>[2x]MSKAFDLVVIGAGSGGLEAGWNAATLYGKRVAVVDVQTSHGPPFYAALGGTCVNVGCVPKKLMVTGAQYMDHLRESAGFGWEFDGSSVKANWKKLIAAKNEAVLDINKSYEGMFNDTEGLDFFLGWGSLESKNVVVVRETADPKSAVKERLQADHILLATGSWPQMPAIPGIEHCISSNEAFYLPEPPRRVLTVGGGFISVEFAGIFNAYKPPGGKVTLCYRNNLILRGFDETIREEVTKQLTANGIEIMTNENPAKVSLNTDGSKHVTFESGKTLDVDVVMMAIGRIPRTNDLQLGNVGVKLTPKGGVQVDEFSRTNVPNIYAIGDITDRLMLTPVAINEGAALVDTVFGNKPRKTDHTRVASAVFSIPPIGTCGLIEEVAAKEFEKVAVYMSSFTPLMHNISGSKYKKFVAKIVTNHSDGTVLGVHLLGDGAPEIIQAVGVCLRLNAKISDFYNTIGVHPTSAEELCSMRTPSYYYVKGEKMEKLPDSNL

T. brucei subspecies, along with all parasites of the order Kinetoplastida, possesses a novel thiol called trypanothione [N1, N8-bis(glutathionyl)spermidine]. Protection of the parasite against oxidative stress is achieved through the oxidation of the dithiol form of trypanothione (T(SH)2) into the disulphide form (T(S)2), followed by regeneration of T(SH)2 by the NADPH-dependent enzyme trypanothione reductase (TryR). However, the enzymes trypanothione reductase and glutathione reductase are highly specific for their respective disulphide substrates such that selective inhibition by small molecules can be readily achieved. Metabolism of trypanothione and other low molecular weight thiols has been established as an attractive target for drug discovery in several trypanosomatids and TryR from T. b. brucei has been specifically validated as a drug target, inter alia, by conditional knockout experiments.

Large crystals (approximately 0.8 mm × 0.3 mm × 0.05 mm) diffracting to 2.3 Å were obtained in drops containing 2.0 μl of protein solution plus 1.0 μl reservoir solution, where the reservoir consisted of 0.1 M bis-Tris propane pH 8.0, 5% PEG 400, 2 M ammonium sulphate. Diffraction data was solved by molecular replacement using the TcTryR structure; the overall statistics of the final TbTryR model are given in Table 4. TbTryR is a homodimer and each subunit of the final model comprises 489 amino acid residues, 1 FAD, 1 NADPH, 4 glycerol and 1 sulphate molecules. Also present are 786 solvent positions that were modelled as oxygen atoms and 1 PEG400 molecule (associated with subunit A). The first residue and the last 2 residues in both subunits were excluded from the structure as there was no convincing electron density to model. The same applies to the nicotinamide moieties of the two NADPH molecules, which were not included in the final model. The overall structure of TbTryR is nearly identical to that of TcTryR (rmsd = 0.6 Å over 482 Cα atoms). All the catalytically important residues (Cys52, Cys57 and His461) and residues interacting with T(S)2, including those involved in binding the spermidine moiety (Leu17, Glu18, Trp21, Met 113, Ser109, Tyr110) are conserved between both structures. Analytical ultracentrifugation indicated 90% of the sample was present at a molecular weight of approximately 93 kDa (data not shown). Both techniques therefore indicated the protein was almost entirely present as a dimer in solution. We have observed no significant differences between the TbTryR and TcTryR in terms of Km, sensitivity to inhibitors or in crystal structure.>HHGIRMTRISREMMKELLSVYFIMGSNNTKADPVTVVQKALKGGATLYQFREKGGDALTGEARIKFAEKAQAACREAGVPFIVNDDVELALNLKADGIHIGQEDANAKEVRAAIGDMILGVAAHTMSEVKQAEEDGADYVGLGPIYPTETKKDTRAVQGVSLIEAVRRQGISIPIVGIGGI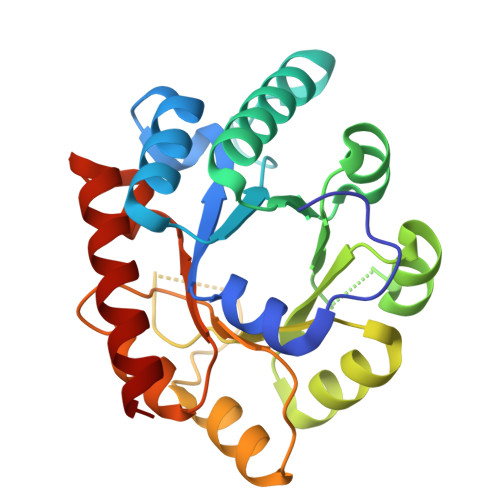TIDNAAPVIQAGADGVSMISAISQAEDPESAARKFREEIQTYKTGR[2x]>GSMSRSKRDNNFYSVEIGDSTFTVLKRYQNLKPIGSGAQGIVCAAYDAILERNVAIKKLSRPFQNQTHAKRAYRELVLMKCVNHKNIIGLLNVFTPQKSLEEFQDVYIVMELMDANLCQVIQMELDHERMSYLLYQMLCGIKHLHSAGIIHRDLKPSNIVVKSDCTLKILDFGLARTAGTSFMMTPYVVTRYYRAPEVILGMGYKENVDIWSVGCIMGEMIKGGVLFPGTDHIDQWNKVIEQLGTPCPEFMKKLQPTVRTYVENRPKYAGYSFEKLFPDVLFPADSEHNKLKASQARDLLSKMLVIDASKRISVDEALQHPYINVWYDPSEAEAPPPKIPDKQLDEREHTIEEWKELIYKEVMDLE[2x];>[2x]YSDDKPFLCTAPGCGRRFTNEDHLAVHKRKHEMTLKFGPA

Activating transcription factor 2 (ATF2) is ubiquitously expressed in most cell types and regulates the transcription of various genes involved in a broad spectrum of cellular functions: cell growth, development and stress. Mitogen-activated protein kinases (MAPK) control transcription by phosphorylating TADs. In the present study, we explore the structural and mechanistic basis of ATF2 regulation by two MAPKs: JNK and p38. We showed that JNK and p38 bind to the ATF2 TAD through distinct regions.

We found that an intact Zn-finger partially overlapping with the D-motif is the minimal JNK binding domain of ATF2. In addition, we set out to determine the crystal structure of the JNK-ATF2 complex using the ATF2(19–58)_Q34R/H47R construct that bound to JNK1 ~100-fold stronger compared to wild-type. The crystal structure showed that M51, L53, and F55 from the ATF2 D-motif bind in the hydrophobic pockets, while K48 binds in the negatively charged CD groove. Zn-finger residues also make contacts to JNK1 and mutations of these (K48, V44, H47 or Q34) greatly affected binding. Furthermore, arginine replacements at position 34 and 47 increased binding by creating additional H-bonds at the JNK:Zn-finger interface. The new crystallographic model provides the structure of the biologically relevant JNK1-ATF2 complex. In addition to making extra contacts, the Zn-finger in the ATF2 TAD contributes to the binding energy by decreasing the entropic cost of binding in the MAPK D-groove. Interestingly, the ATF2_CACA construct (in which the Zn-finger structure is disrupted) bound p38 better compared to wild-type while JNK binding decreased. This suggests that the Zn-finger limits the capacity of the partially overlapping D-motif to bind to p38 and favors JNK binding. The Zn-finger+D-motif module is more JNK-specific compared to an NFAT4-type D-motif, and specificity is achieved through both positive and negative factors that promote JNK- and limit p38-binding, respectively.> KETAAAKFERQHMDSSTSAASSSNYCNQMMKSRNLTKDRCKPVNTFAHESLADVQAVCSQKNVACKNGQTNCYQSYSTMSITDCRETGSSKYPNCAYKTTQ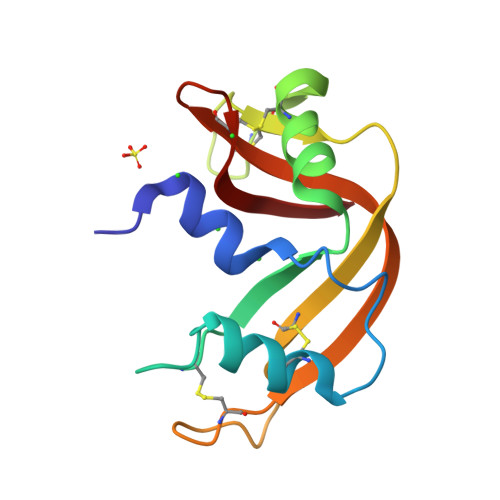ANKHIIVACEGNPYVPVHFDASV>LEFPGAEGQWTRFPKWNACCESEMSFQLKTRSARGLVLYFDDEGFCDFLELILTRGGRLQLSFSIFCAEPATLLTDTPVNDGAWHNVRIRRQFRNTTLFIDQVEAKWVEVKSKRRDMTVFSGLFVGGLPPELRAAALKLTLASVREREPFKGWIRDVRVNSSLALPVDSGEVKLDDEPPNSGGGSPCEAGEEGEGGVCLNGGVCSVVDDQAVCDCSRTGFRGKDCSQGKEEYIATFKGSEYFCYDLSQNPIQSSSDEITLSFKTLQRNGLMLHTGKSADYVNLALKNGAVSLVINLGSGAFEALVEPVNGKFNDNAWHDVKVTRNLRQVTISVDGILTTTGYTQEDYTMLGSDDFFYVGGSPSTADLPGSPVSNNFMGCLKEVVYKNNDVRLELSRLAKQGDPKMKIHGVVAFKCENVAT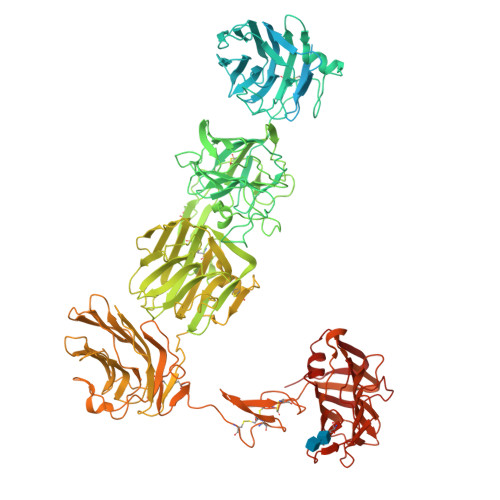LDPITFETPESFISLPKWNAKKTGSISFDFRTTEPNGLILFSHGKPRHQKDAKHPQMIKVDFFAIEMLDGHLYLLLDMGSGTIKIKALQKKVNDGEWYHVDFQRDGRSGTISVNTLRTPYTAPGESEILDLDDELYLGGLPENKAGLVFPTEVWTALLNYGYVGCIRDLFIDGQSKDIRQMAEVQSTAGVKPSCSRETAKPCLSNPCKNNGMCRDGWNRYVCDCSGTGYLGRSCEREATVLSYDGSMFMKIQLPVVMHTEAEDVSLRFRSQRAYGILMATTSRDSADTLRLELDAGRVKLTVNLDCIRINCNSSKGPETLFAGYNLNDNEWHTVRVVRRGKSLKLTVDDQQAMTGQMAGDHTRLEFHNIETGIITERRYLSSVPSNFIGHLQSLTFNGMAYIDLCKNGDIDYCELNARFGFRNIIADPVTFKTKSSYVALATLQAYTSMHLFFQFKTTSLDGLILYNSGDGNDFIVVELVKGYLHYVFDLGNGANLIKGSSNKPLNDNQWHNVMISRDTSNLHTVKIDTKITTQITAGARNLDLKSDLYIGGVAKETYKSLPKLVHAKEGFQGCLASVDLNGRLPDLISDALFCNGQIERGCEGPSTTCQEDSCSNQGVCLQQWDGFSCDCSMTSFSGPLCNDPGTTYIFSKGGGQITYKWPPNDRPSTRADRLAIGFSTVQKEAVLVRVDSSSGLGDYLELHIHQGKIGVKFNVGTDDIAIEESNAIINDGKYHVVRFTRSGGNATLQVDSWPVIERYPAGRQLTIFNSQATIIIGGKEQGQPFQGQLSGLYYNGLKVLNMAAENDANIAIVGNVRLVGEVPSASTSHHHHHH[2x]> AEVAPGDVAIDGQGHVARPLTDAPGDPVEGRRLMTDRSVGNCIACHEVTEMADAQFPGTVGPSLDGVAARYPEAMIRGILVNSKNVFPETVMPAYYRVEGFNRPGIAFT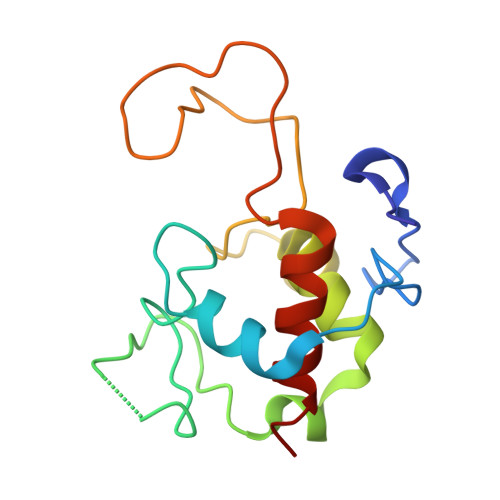SKPIEGEIRPLMTAGQIEDVVAYLMTLTQ We identified PBI1 (PUB44-INTERACTING 1), which belongs to a protein family with the DUF1110 domain. PBI1 interacts with WRKY45 and negatively regulates its activity. Therefore, it appears that PBI1 keeps WRKY45 in an inactive state in the absence of pathogen attack, and that PUB44-mediated degradation of PBI1 activates immunity via the de-suppression of WRKY45. PBI1 is degraded upon perception of chitin, and this is suppressed by silencing of PUB44 or expression of XopP, indicating that PBI1 degradation depends on PUB44.

Although PBI1 consists mainly of the DUF1110 domain, the molecular nature of this domain was unknown. Therefore, we determined its tertiary structure of PBI1. The crystal structure was solved at a resolution of 1.84 Å. PBI1 is composed of a four-helix bundle with a diameter of approximately 19 Å and a length of about 70 Å. There are six molecules in the asymmetric unit. The root mean square differences (r.m.s.d.) between each monomer are from 0.15 to 0.85 Å. We observed no large conformational change induced by crystal packing. The four helices of PBI1 are arranged in an up-down-up-down topology, and the bundle is leftward turning. The interfaces between the helices consist of hydrophobic residues, whereas hydrophilic residues are exposed on the surfaces that interact with the aqueous environment. In particular, the CC domain of Rx is very similar in structure to PBI1, with a high Z-score of 4.5.

>[6x]GPGHMMAAEAWRSRFRERVVEAAERWESVGESLATALTHLKSPMHAGDEEEAAAARTRIQLAMGELVDASRNLASAMSLMKVAELLALHGGSVNPSTHLGEISLLGDQYLAERNAGIKLLEAGKDARKAYISVDGCRGNLDAILLLLDHPRVPCVDDFIEEELFVAGDNLQGAIGNAKLGTERAVGARQDVSGAN> GVVKFDIKNQCGYTVWAAGLPGGGKRLDQGQTWTV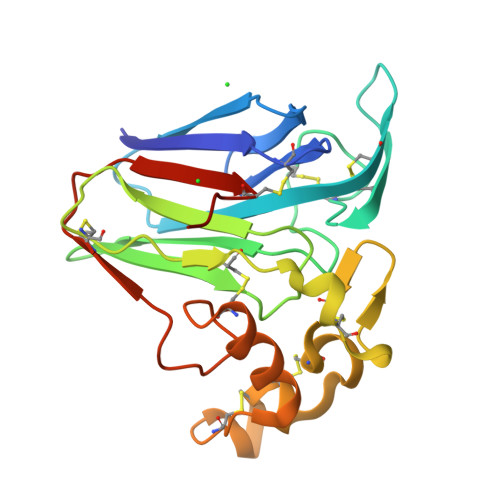NLAAGTASARFWGRTGCTFDASGKGSCQTGDCGGQLSCTVSGAVPATLAEYTQSDQDYYDVSLVDGFNIPLAIQPTNAQCTAPACKADINAVCPSELKVDGGCNSACNVFKTDQYCCRNAYVDNCPATQYSKIFKNQCPQAYSYAKDDTATFACASGTDYSIVFCPHHHHHH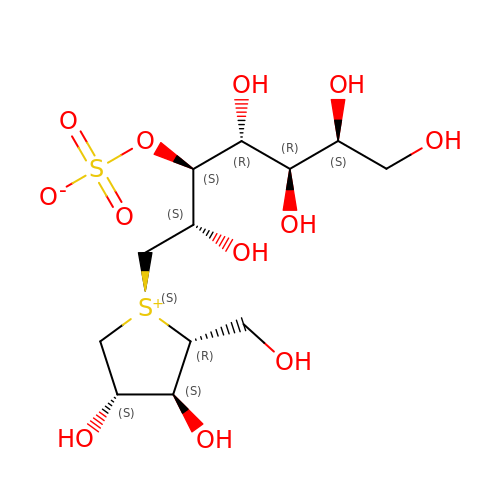(1S,2R,3R,4S)-1-{(1S)-2-[(2R,3S,4S)-3,4-dihydroxy-2-(hydroxymethyl)tetrahydrothiophenium-1-yl]-1-hydroxyethyl}-2,3,4,5-tetrahydroxypentyl sulfate | C12 H24 O12 S2 | OMKXVFDVAGCPBS-QTIKZJLFSA-N> MENLSDVFDIYAICACCKVAPTSAGTKNEPFSPRTFRGLGNKGTLPWKCNSVDMKYFSSVTTYVDESKYEKLKWKRERYLRMEASQGGGDNTSGGDNTHGGDNADKLQNVVVMGRSSWESIPKQYKPLPNRINV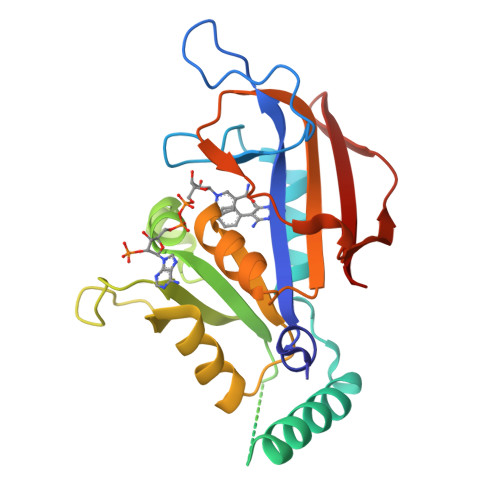VLSKTLTKEDVKEKVFIIDSIDDLLLLLKKLKYYKCFIIGGAQVYRECLSRNLIKQIYFTRINGAYPCDVFFPEFDESEFRVTSVSEVYNSKGTTLDFLVYSKV alpha-D-psicofuranose 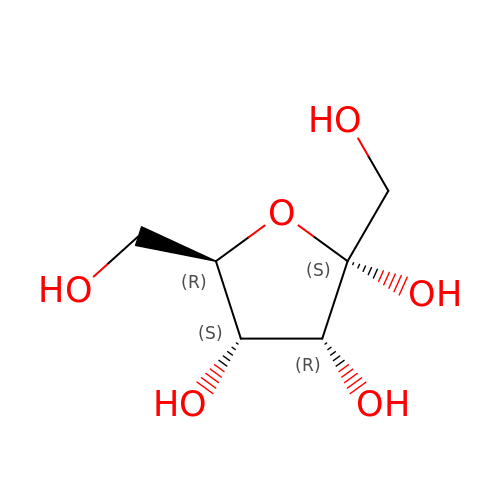| C6 H12 O6 | RFSUNEUAIZKAJO-KAZBKCHUSA-N> MNRTGGSIYAHALSQFAVCRQPWNEYIGLLTKQDSTPYHTEPQEKPAYRGRKQGREGWLFGQQVQLHYHRFPDEQLITNLSRWRTGETVGDIAMQQFRNAQPFDIEDKDPQGVQRPSPEVYMKLNYKNPATISRFLTRTGHMYPADILPLNP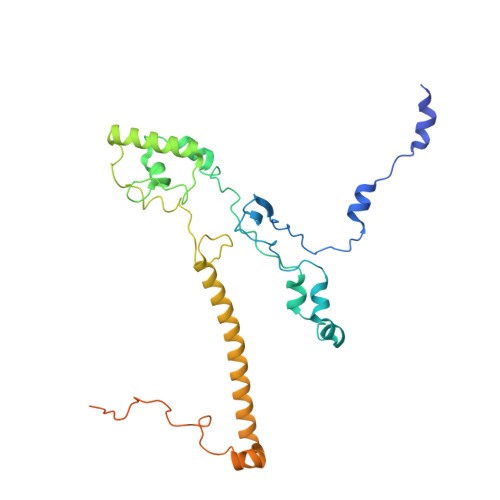EAVVKLRVAKAQAIRIGLYPRFGNPFWFRSQKFRPKAYQENYDPTTYSTKRTVEHFAYNWVQTDRIRRYFRELEAVHTSGSASARGSGGGTTAEHKQQDQFYSPENQPISLHRNNISYMEDVGRSVKNPTVPGLMSTKGMKKKFHNLYSSTSTKRMGFSNPTLGIKKV>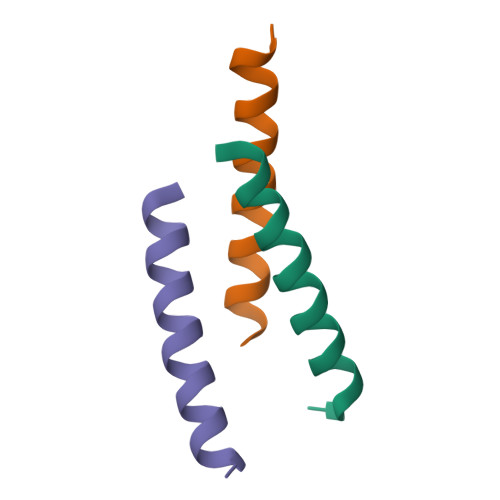[39x]GPMEEQREILEQLKKTLQMLTVEL>[6x]MAHHHHHHADTLSDVKAKGFLQCGVNTGLLGFASPNDKGEWSGFDVDYCRAVASAIFGDPTKVKFTPLNAKERFTALQSGEVDVLIRNTTWTISRDTSLGLDFAGINYYDGQGFMINSKKLAGINSALQLSGASICVQAGTTTELNMADYFRAN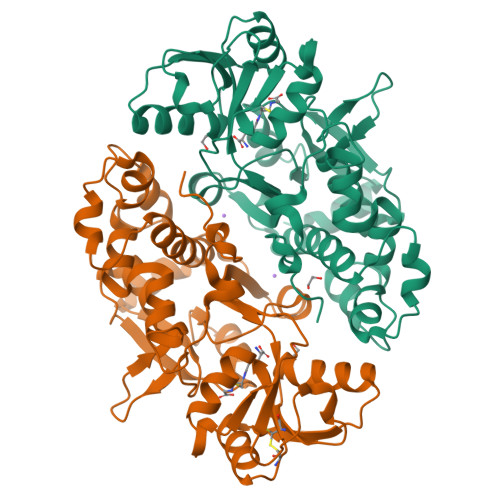KMEYNPVVFEKIEEANAAYDSGRCDAYTTDQSSLYGVRLALANPDDHVILPEIISKEPFGLTVRQGDARWADVVRWTHNALLNAEEYGITQANVEEMKKSDNPDIKRLLGAEADTKIGTDLGLDKDWVVKIIKGVGNYGEIFERNIGSGSPLKIARGLNAQWNKGGLQYGIPVR>[4x]SNELKVREFYRLHNACVKLK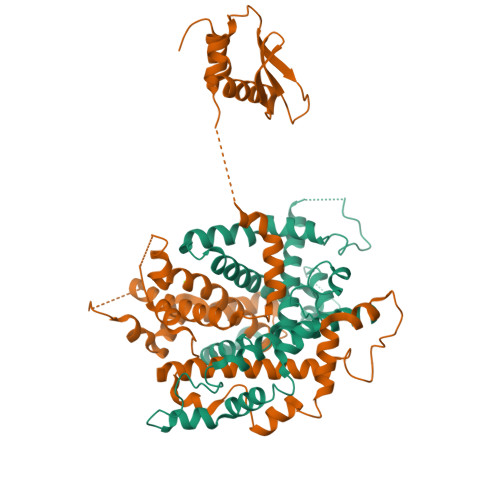ESIKLIYENPLVTDQNVLNLGTAENTIDYTILNTPTLNVAKTLLGNRYSLDLIDLFQSHDFKDSNTDVDMFIKYPVVYDENLENLAFMHKSFPNMNAHLNDAQKTQLSNERLEFLGDSWLGALVSYIVYTRFPSANEGMLSQMKESIVNNNNLFDWSTKLNFTKRLQGNIATPTRVVKDKMSKRYADCVEAYIGALVIDRFGTEFLDIKEWLEELSEKKLAKSSQMVIKEPLNKNAKNELAELLQINKLGHKLHYRKLTEMPPFRVEVKIGDILLDEAEGNSIREAEHRAAMKVLENDELLRKYSVYDLEDGNSKKYSIEE> SDELYRQSLEIISRYLREQATGAKDTKPMGRSGATSRKALETLRRVGDGVQRNHETAFQGMLRKLDIKNEDDVKSLSRVMIHVFSDGVTNWGRIVTLISFGAFVAKHLKTINQESCIEPLAES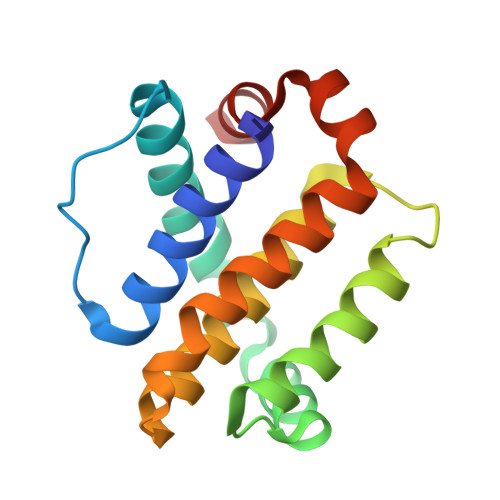ITDVLVRTKRDWLVKQRGWDGFVEFFHVE>AHYNTEILKSIDNEWRKTQCMPREVAIDVGKEFGVATNTFFKPPCVSVYRCGGCCNSEGLQCMNTSTSYLSKTLFEITVPLSQGPKPVTISFANHTSCRCMSKLHHHHHH[4x];>DYRSPFIASVSDQHGVVYITENKNKTVVIPCLGSISNLNVSLCARYPEKRFVPDGNRISWDSKKGFTIPSYMISYAGMVFCEAKINDESYQSIMYIVVVVGYRIYDVVLSPSHGIELSVGEKLVLNCTARTELNVGIDFNWEYPSSKHQHKKLVNRDLKTQSGSEMKKFLSTLTIDGVTRSDQGLYTCAASSGLMTKKNSTFVRVHED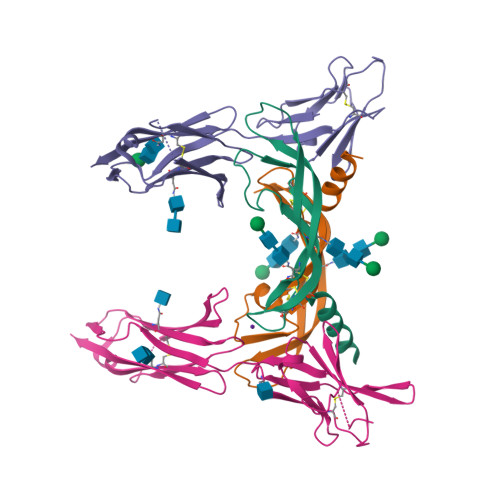PIEGR[4x]>[6x]MSRSIAQMIDHTLLKPNTTEDQIVK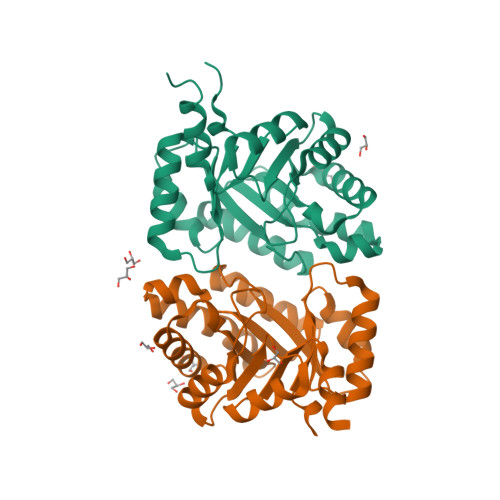LCEEAKEYSFASVCVNPTWVALAAQLLKDAPDVKVCTVIGFPLGATTPEVKAFETTNAIENGATEVDMVINIGALKDKQYELVGRDIQAVVKAAEGKALTKVIIETSLLTEEEKKAACELAVKAGADFVKTSTGFSGGGATAEDIALMRKVVGPNLGVKASGGVRDLSDAKAMIDAGATRIGASAGVAIVNGERSEGSY> GAMAAKFRASNIMPSSSFHMSPTSNEDLRKIPDSNPFDATAGYRSLTYEEVLQELVKHKELLRRKDTHIRELEDYIDNLLV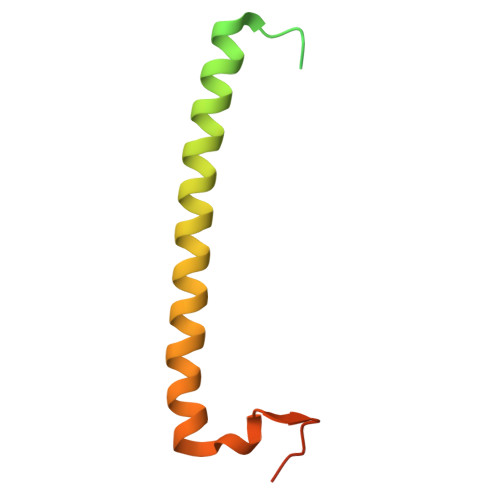RVMEETPSILRVPYEPSRKAGKFSNS Our comparative bioinformatics studies suggest that among those reported as glycosyltransferases are also pseudo-glycosyltransferases (such as VldE, EC 2.x.x.x), which do not recognize sugars as substrates but rather catalyze the formation of non-glycosidic C-N bonds in the biosynthesis of C7N-aminocyclitol-containing natural products such as acarbose and validamycin A. Validoxylamine A is generated through the dephosphorylation of validoxylamine A 7′-phosphate by VldH while validoxylamine A 7′-phosphate (VDO) results from a condensation of GDP-valienol and validamine 7-phosphate (both are pseudo-sugars) by the pseudo-glycosyltransferase, VldE. Similar to OtsA, VldE is comprised of two Rossman β/α/β domains which are oriented in a GT-B configuration. As was described in a recent crystallographic study of ValL, a VldE homolog from S. hygroscopicus subsp. jinganggensis, VldE is a homodimer.

The first crystallographic structure of VldE in complex with the entirety of its products, VDO and GDP, was elucidated. Surprisingly, the structure of VldE in complex with the entirety of its products (VldE•GDP•VDO), GDP and VDO was also in an open conformation and a comparison to the VldE•GDP model showed that the binding of VDO also did not have an effect of the global conformation of VldE (RMSD Cα = 0.262 Å). The hydroxyls of the donated cyclitol make numerous interactions with the backbone amides of VldE at residues Gly384, Gln385, Asn386, and Leu387. The donated cyclitol also makes interactions with the side-chains of residues His182 and Asp383. Also conserved is the interaction of the β-phosphate with the formerly bound carbon of the donated cyclitol. Asp158 swings 62–83° towards the catalytic center in recognition of the hydroxyls of the acceptor cyclitol. Upon the binding of the phosphorylated acceptor group, the guanidine moiety of Arg326 enters into an interaction with the phosphate oxygens. This interaction allows Tyr159 to swing 110–112° to make an interaction with Arg326. Within the VldE•GDP•VDO model, Arg326 and Asn325 interact with the phosphorylated cyclitol and most likely help to ensure the proper position of validamine 7-phosphate for catalysis. Despite the conservation of the interactions between the catalytic site and VDO, there is no observed conformational closing of the catalytic site upon the binding of the acceptor cyclitol as was witnessed in structural studies of OtsA.

>[2x]MTGSEIFLASKRAAITYDTDPATGEPRAWLAPGGTGNVVAEQAGVLNISWIASADSEDDRRASALNPDGVTMELHSGREILVRLIRHDPAVFRNVQNFMTANLMWAANNYGWDRWTQPSFGSDAREGWADFGRFTRDFADAILKSSAQSADPVYLVHDYQLVGVPALLREQRPDAPILLFVHIPWPSADYWRILPKEIRTGILHGMLPATTIGFFADRWCRNFLESVADLLPDARIDREAMTVEWRGHRTRLRTMPLGYSPLTLDGRNPQLPEGIEEWADGHRLVVHSGRTDPIKNAERAVRAFVLAARGGGLEKTRMLVRMNPNRLYVPANADYVHRVETAVAEANAELGSDTVRIDNDNDVNHTIACFRRADLLIFNSTVDGQNLSTFEAPLVNERDADVILSETCGAAEVLGEYCRSVNPFDLVEQAEAISAALAAGPRQRAEAAARRRDAARPWTLEAWVQAQLDGLAADHAARTATAERFDTAPAVSTRADL>VTAYEEIVCQVFAAVLDRSDVTADADFFALGGHSLLSLRVVARLRALLGVDVGVRDLFEAPTPAALAARLTTQTGRRPAVTRRGPDAPPVLSHFQRRLWLIEQVYQTRGAYNVPLAVHVSDRLDLDVLRAAVRDLVARHEVLRTLVRSSDDGPDPVLLAPEDAAVDVAEVQAAGPVADLLAELTAQPFDLATQ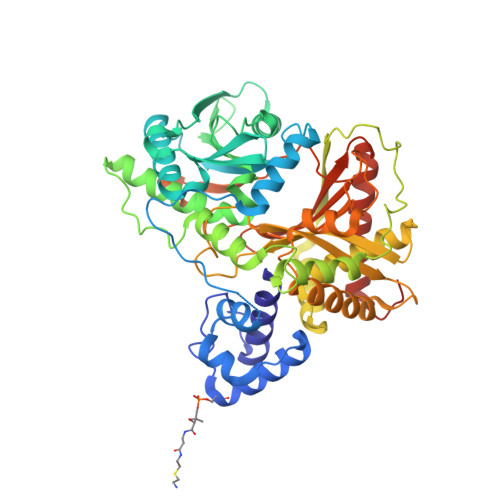IPLRVRMITGEQVDGCVLLLVCHHIAADEWSFAPLLRDLDTAYRARAAGRAPDWEPLPAQYSDYAATLHDWLGEATDPASPLRRQLDYWQHALQDLPDELDLPTDRPRPATASHRGGLARAELPPELVEAVRRLAAQHGVTVFMVVQAAVAVLLHRLGAGDDIPLGSPVADRADEAVHDTVGFFLNTLVLRVNLSGNPTFADLLDRVRAVDLEAFARADAPFDAVVDTVKPPRAVSRHPLFQTMVSYQRRPSDVDRLFGAATRLVEVPLDTAKFDLEFAFIEDGHGGAHIALNYAADLFDHDSAEQLVARLRTVLEHACADPCRPVAGVEVVSGA[2x]5-({6-[(piperidin-4-ylmethyl)amino]pyrimidin-4-yl}amino)pyrazine-2-carbonitrile | C15 H18 N8 | 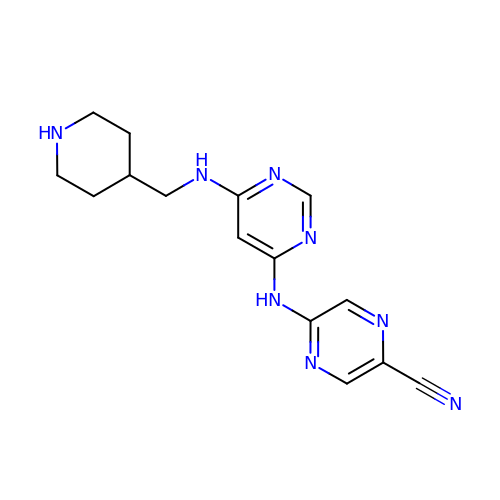LNWARQATROLGJR-UHFFFAOYSA-N6-ammonio-N-(trifluoroacetyl)-L-norleucyl-N-[4-(trifluoromethyl)phenyl]-L-alaninamide | C18 H23 F6 N4 O3 | 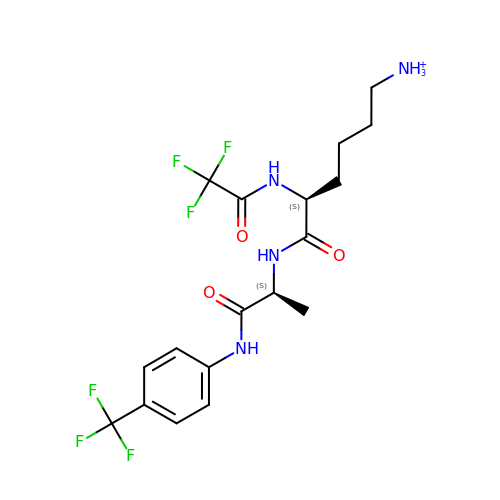HGUBHDYUXLPGND-GWCFXTLKSA-O> GPKLKGRKIVGGKAEGEVIVSRKPLSFLGGVDPETGIVTDAESDIRGQSIAGKILVF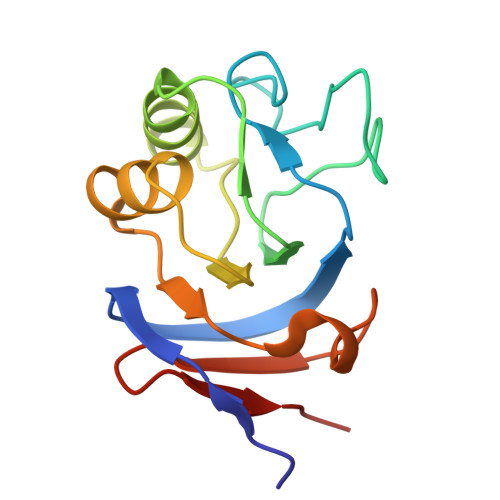PRGKGSTVGSYVIYALKKNNKAPKAIIVGEAETIVATGAIISDIPMVDGVDVSKLKTGMKVRVDADSGEVEILEDGE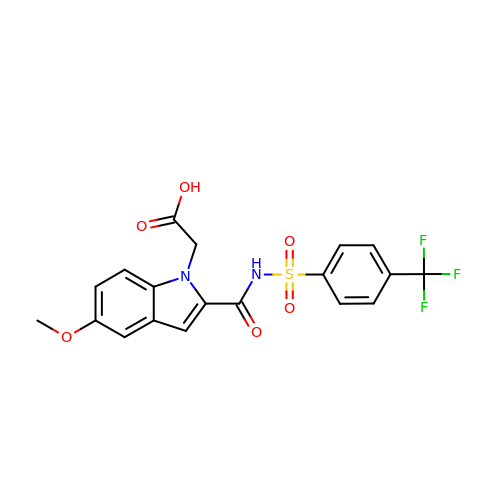[5-methoxy-2-({[4-(trifluoromethyl)phenyl]sulfonyl}carbamoyl)-1H-indol-1-yl]acetic acid | C19 H15 F3 N2 O6 S | DLVZBWPTLGVTNH-UHFFFAOYSA-N> MLDSKLNNIRFETISSKYYDDVIEHLRQTFFADEPLNKAVN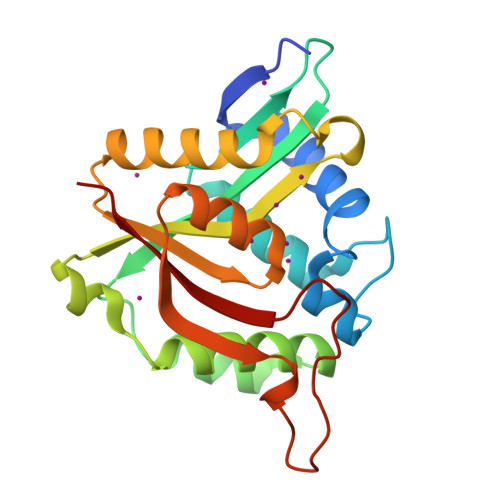LTRPGQGHPLLEQHSLSTLKDNVSIMAISNDGDIAGVALNGILYGNTDIEKSREKLNEIQDESFKKIFKLLYEQNLKINLFKQFDVDKIFEIRILSVDSRFRGKGLAKKLIEKSEELALDRGFQVMKTDATGAFSQRVVSSLGFITKCEINYTDYLDENGEQIFVVDPPHEKLKIMCKVIN>[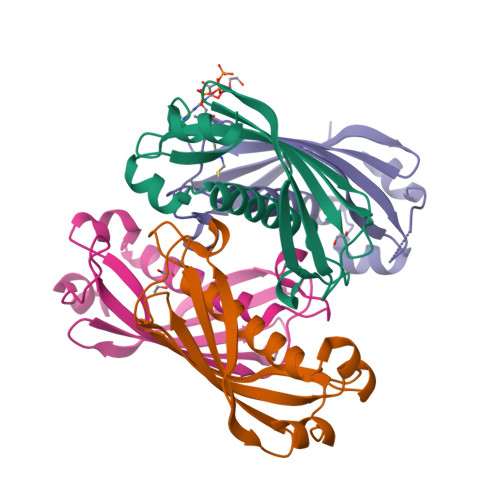4x]VNTTLFRWPVRVYYEDTAAGGVVYHASYVAFYERARTEMLRHHHFSQQALMAERVAFVVRKMTVEYYAPARLDDMLEIQTEITSMRGTSLVFTQRIVNAENTLLNEAEVLVVCVDPLKMKPRALPKSIVAEFKQ>[2x]MNTVSPAKKKVIIIGAGIAGLKAASTLHQNGIQDCLVLEARDRVGGRLQTVTGYQGRKYDIGASWHQDTLTNPLFLEEAQLSLNDGRTRFVFDDDNFIYIDEERGR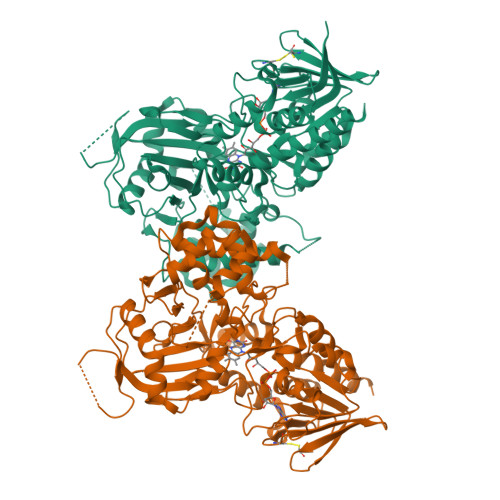VDHDKELLLEIVDNEMSKFAELEFHQHLGVSDCSFFQLVMKYLLQRRQFLTNDQIRYLPQLCRYLELWHGLDWKLLSAKDTYFGHQGRNAFALNYDSVVQRIAQSFPQNWLKLSCEVKSITREPSKNVTVNCEDGTVYNADYVIITVPQSVLNLSVQPEKNLRGRIEFQPPLKPVIQDAFDKIHFGALGKVIFEFEECCWSNESSKIVTLANSTNEFVEIVRNAENLDELDSMLEREDSQKHTSVTCWSQPLFFVNLSKSTGVASFMMLMQAPLTNHIESIREDKERLFSFFQPVLNKIMKCLDSEDVIDGMRPIENIANANKPVLRNIIVSNWTRDPYSRGAYSACFPGDDPVDMVVAMSNGQDSRIRFAGEHTIMDGAGCAYGAWESGRREATRISDLLKLEHHHHHH> PGSMPVRPDLQQLEKCIDDALRKNDFKPLLALLQIDICEDVKIKCSKQFLRKLDDLICRELNKKDIQTVSSILISIGRCSKNIFILGQAGLQTMIKQGLVQKMVSWFENSKEIILNQQQSKDEAVMNMIEDLFDLLMVIYDISDEGKNQVLESFIPQI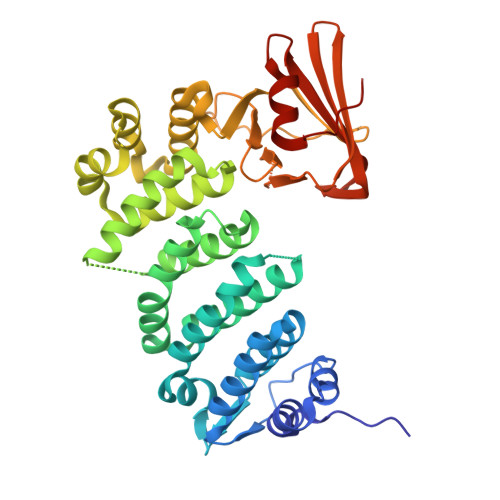CALVIDSRVNFCIQQEALKKMNLMLDRIPQDANKILSNQEMLTLMSNMGERILDVGDYELQVGIVEALCRMTTEKRRQELAYEWFSMDFIANAFKEIKDCEFETDCRIFLNLVNGILGDKRRVYTFPCLSAFLGKYELQIPSDEKLEEFWIDFNLGSHTLSFYIAGDEEDHQWEAVTVPEEKVQMYNIEVRESKKLLTLTLKNIVKISKKEGKELLFYFDESLEITNVTKKVFGGLEHHHHHH>DILECDYFDTVDISAAQKLQNGSYLFEGLLVPAILTGEYDFRILPDDSKQKVARHIRGCVCKLKPCVRFCCPH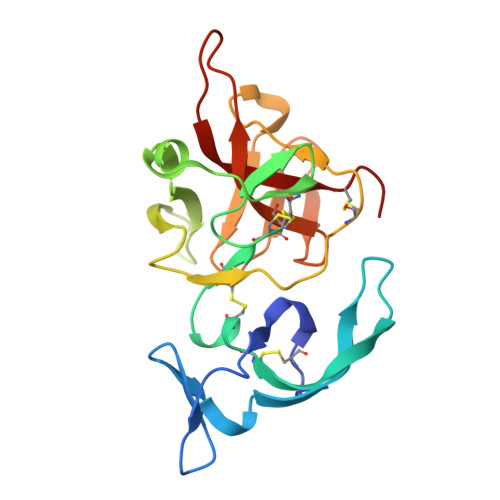DHIMDNGVCYDNMSDEELAELDPFLNVTLDDGSVSRRHFKNELIVQWDLPMPCDGMFYLDNREEQDKYTLFENGTFFRHFDRVTLRKREYCLQHLTFADGNATSIRIAPHNCLIV[4x]> KHKILHRLL;> PVERILEAELAVEPKTETYVEANMGLNPSSPNDPVTNICQAADKQLFTLVEWAKRIPHFSELPLDDQVILLRAGWNELLIASFSHRSIAVKDGILLATGLHVHRNSAHSAGVGAIFDRVLTELVSKMRDMQMDKTELGCLRAIVLFNPDSKGLSNPAEVEALREKVYASLEAYCKHKYPEQPGRFAKLLLRLPALRSIGLKCLEHLFFFKLIGDTPIDTFLMEML;> HKPEPTDEEWELIKTVTEAHVATNAQGSHWKQKRKFLPEDIGQAPIVNAPEGGKVDLEAFSHFTKIITPAITRVVDFAKKLPMFCELPCEDQIILLKGCCMEIMSLRAAVRYDPESETLTLNGEMAVTRGQLKNGGLGVVSDAIFDLGMSLSSFNLDDTEVALLQAVLLMSSDRPGLACVERIEKYQDSFLLAFEHYINYRKHHVTHFWPKLLMKVTDLRMIGACHASRFLHMKVECPTELFPPLFLEVFED

NRs harbour a C-terminal ligand-binding and transactivation domain (LBD), a central DNA-binding domain and a variable N-terminal disordered transactivation domain. A subset of NRs functions as heterodimers with retinoid X receptor (RXR), and thus provides a mechanism to integrate two distinct ligand signalling pathways. Second, RXR heterodimers that contain retinoic acid receptor (RAR), vitamin D receptor (VDR) or thyroid hormone receptor (TR), are ‘non-permissive' for RXR as they generally do not respond to RXR ligands, or do so only in certain contexts in the presence of the partner ligand. Here we present comprehensive structural analyses of a ‘permissive' (PPARγ/RXRα) and ‘non-permissive' (TR/RXR) heterodimeric complex, which defines how a non-permissive dimer partner allosterically silences RXR.

To further detail the structural mechanism by which TRβ allosterically silences RXRα, we crystallized apo-RXRα in complex with TRβ, T3 and a co-activator peptide derived from SRC-2. The anisotropic data set was scaled to a resolution of 3.2–3.8 Å and refined to an Rwork/Rfree of 23.6/28.1%. Consistent with other RXR heterodimer structures, TRβ and RXRα interact via the conserved dimer interface, largely comprised of helix 11 in each monomer, with additional contacts from helices 8 and 10. TRβ adopts the active conformation when bound to T3, with helix 12 forming one side of the co-activator-binding site, allowing the docking of the SRC-2 peptide. RXRα displays an inactive conformation with no bound ligand or co-activator peptide while helix 12 docks at the AF-2 surface. Although the asymmetric unit of the TRβ·T3/apo-RXRα complex is a dimer, the crystal packing reveals a heterotetramer assembly. Compared with other RXR dimers fully occupied by ligands—including the RXRα homodimer46, and permissive RXR heterodimer complexes with LXR47 and PPARγ48—our structure of the TRβ·T3/apo-RXRα heterodimer shows a marked shift in TRβ helix 11. This shift induces a rotation of RXRα helix 11, which is visualized by comparing our TRβ·T3/apo-RXRα heterodimer with the RXRα homodimer or with the apo-RXRα tetramer. Notably, the TRβ-directed rotation of RXRα helix 11 in the TRβ·T3/apo-RXRα structure induces a corresponding rotation of the adjacent RXR helix 5, which in turn disrupts the active conformation of RXRα. In contrast, in the TRβ·T3/apo-RXRα structure TRβ-induced rotation of RXRα helix 5 in the heterodimer provokes a clash with the active conformation of helix 12 that pushes both L276 in helix 3 and M454 in helix 12 away from W305 in helix 5.>[4x]GPGSEFELRRQASNYQLTLTNTRATVNILMERLKKSDADVEQYRAELESVQLAKGALEQSYLVLQADAEQLRQQLTESQDALNALRSSSQTLQSE;>GPGSMKEQLLYLSKLLDFEVNFSDYPKGNHNEFLTIVTLSTHPPQICHGVGKSSEESQNDAASNALKILSKL[4x]

Mira is a key adaptor protein that directs several cell fate determinants to basal cortex during the asymmetric division of Drosophila NB. Mira is a multi-domain scaffold protein that concentrates at the basal cortex along with its cargos during mitosis of Drosophila NB asymmetric division. The Stau family of dsRNA-binding proteins exerts a conserved function in mRNA transport, localization and translational control from Drosophila to mammals. However, both dsRBDs 2 and 5 are required for the anchoring of bicoid mRNA, whereas dsRBD5 also directs the actin-dependent localization of pros mRNA through interaction with Mira, pointing to other functional roles of dsRBDs 2 and 5 rather than RNA binding.

The complex structure was solved by single-wavelength anomalous dispersion using Se–Met derivatives at 2.5 Å resolution. The structure revealed that the complex forms a 2:2 heterotetrameric architecture, in which two Stau dsRBD5s interact symmetrically with the N-terminal end of the Mira coiled-coil homodimer. In accord with the previous small-angle X-ray scattering-based structure prediction, two Mira514–595 fragments, each made up of a single contiguous α-helix, dimerize in a parallel manner to form an elongated ‘rod-like' structure. Interestingly, the Mira coiled-coil dimer is slightly asymmetric, with one curved helix A wrapping around the other approximately straight one A′. The two α-helices of Mira514–595 form a quite tight supercoil with an average interhelical distance ∼5.8 Å, a value that is much lower than expected for a canonical coiled-coil (∼9.6 Å). The interesting feature of the Mira514–595/Stau dsRBD5 complex structure is that Stau dsRBD5 binds to Mira through the exposed face of its β-sheet, a mode that has never been observed in any other dsRBDs before this study. Hydrophobic residues, such as Tyr971Stau on β1, Leu980Stau and Ile982Stau on β2, Ile992Stau and Val996Stau on β3 of dsRBD5, Ile528Mira and Leu529Mira from helix A, and Val526′Mira, Met530′Mira, and Leu533′Mira from helix A′ form the hydrophobic core at the interface. Arg532Mira from helix A forms an extensive hydrogen bond network with the side chain of His976Stau, and main chain carbonyls of Pro972Stau and Glu978Stau at L2 of dsRBD5. In agreement with the solved crystal structure, SEC and ITC experiments showed that mutations on Mira (L529E, M530E and R532A) or Stau (Y971K, H994E and I982A) from the Mira–Stau packing interface disrupted or severely impaired the interaction between Mira514–595 and dsRBD5. In line with the complex structure, L557EMira mutation was also found to disrupt the Mira–Stau interaction, demonstrating that the dimer assembly of Mira CBD is crucial for Stau dsRBD5 binding.>MRVTVYGFGSLNYYSNKLNVPEKLGGEPPYGGSAMAVEFAKAGHDVTLSDPNIDKVPDEIRKKVEDAGVKLTTDDIEAAKEAEVAILFTPFRGGVTFKIAETILPYLVENAVICTTCTMSILVLNSYLQNAIFLEGREDIGFSTMHPAAIPGTPQHKHYLIATNELLRKPIVTEEQIEKLKKLATDTGKEAYLLPAELVSPVGDMGIVTTAIAFAGAIEYYKVSRDILKTKRSMTEFQIAQSLQVISSLVTKYGLEGLIKLLNV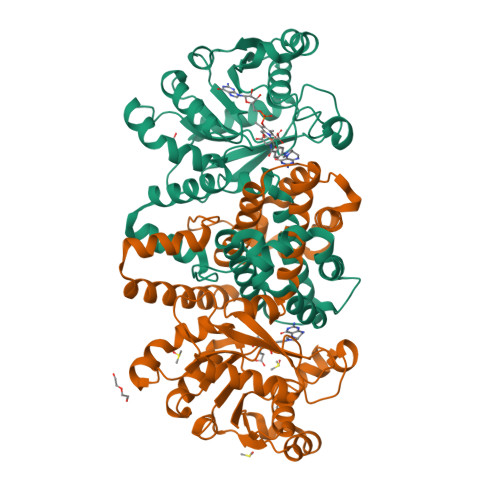DAMKASLQSMILDKNEQPLTVTASKLLEKIEETIPELIKEAENFSPSEPTYTSAPSPMLVEHMEDLVGDDVLKGILRESWKKFYENVSERNKEKLAAALEHHHHHH[4x]Using X-ray crystallography, we show that the ciliopathy-associated centriolar protein CEP120 contains three C2 domains. CEP120, for example, plays a key role in the duplication, elongation, and maturation of centrioles, which in principle could impact the production of a functional basal body (Comartin et al., 2013, Lin et al., 2013, Mahjoub et al., 2010, Wu et al., 2014). All three C2 domains of CEP120 (C2A, C2B, and C2C) adopt the PLC δ1-like topology II and are structurally similar to each other (root-mean-square deviation [RMSD], 2.4–2.6 Å), with major differences found mainly in their loop length. Thus, the CEP120 C2 domains probably play a role as protein-protein interaction modules.

For the O.n.-A200P mutant (equivalent to the H.s.-A199P JATD mutation), we obtained diffraction-quality crystals that allowed a successful structure determination to a resolution of 2.1 Å. To obtain this crystal form, we introduced an additional mutation (G307S) that we found serendipitously. The CEP120 C2B (H.s.-A199P) mutant structure revealed an overall preservation of the C2 domain fold and only subtle structural changes. In the WT structure, the O.n. A200 residue is located at the end of β strand 1 and its side chain points inward toward the hydrophobic interior of the domain. The replacement of this alanine by proline causes a change in the main-chain dihedral angles of the preceding residues, resulting in a local structural change. In the WT structure, the main-chain carbonyl O of O.n.-Phe199 (H.s.-Phe198) makes a main-chain/main-chain hydrogen bond to O.n.-Gly333 (H.s.-Gly333) that cannot be maintained in the A199P mutant due to the conformational constraints imposed by the adjacent proline residue. In the mutant structure, the loss of this hydrogen bond is compensated by a peptide bond flip, allowing the main-chain carbonyl O of O.n.-Ala198 (H.s.-Ala197) to form a new hydrogen bond with O.n.-Gly333 (H.s.-Gly333). The most significant conformational change is observed for O.n.-F244 (H.s.-F243), the side chain of which moves to avoid a steric clash with the bulky pyrrolidine ring of the proline. Other structural differences between the WT and A200P mutant, in particular the conformational change in loop 1 and loop 3, are most likely caused by different crystal-packing interactions.

>GPHMPEKLEAILIPDQGYHQVGPADLCTDMFVLSVTVAFPTKLEQLVPSTMKLSAEGSEFFFYYSLLGNDITSEPFHNLLSPDFEPERASVRIRSSKQILKAFLSQQPSLQIHLCCGNHSLGSTDVSLSALAGISTDLDNKAATVESAFILQPPKRVKQTLPALPTDLQPTLGVAVTLRREEVALQQSVGNKE[2x]>[2x]GSAPVSIWSRVVQFGTGWGFWVSGHVFITAKHVAPPKGTEIFGRKPGDFTVTSSGDFLKYYFTSAVRPDIPAMVLENGCQEGVVASVLVKRASGEMLALAVRMGSQAAIKIG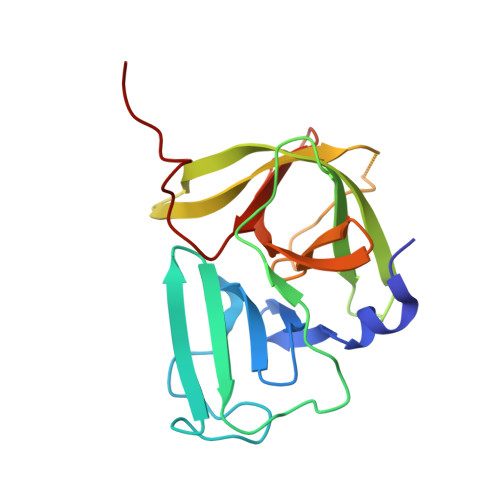SAVVHGQTGMLLTGSNAKAQDLGTIPGDAGCPYVYKKGNTWVVIGVHVAATRSGNTVIAATHGEPTLEALEFQ> NYLDLFSHKNMKLKERVLIPVKQYPKFNFVGKI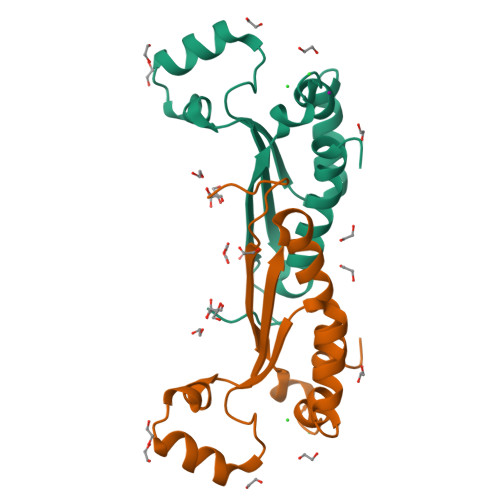LGPQGNTIKRLQEETGAKISVLGKGSMRDKAKEEELRKGGDPKYAHLNMDLHVFIEVFGPPCEAYALMAHAMEEVKKFLVPDM> MGSSH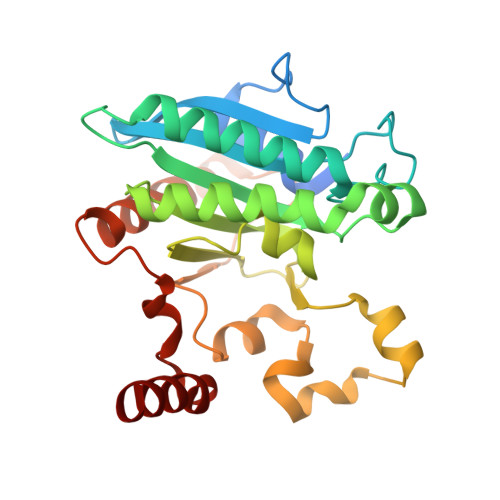HHHHHSQDPNSMSQPFASRGLAWFQALAGSLAPRPGDPASLRVADAELDGYPVRFLAVVPDPDNPFPRARQGEVGLLEGWGLAAAVDEALEADREAPRKRALLAIVDVPSQAYGRREEALGIHQALAGAVDAYARARLAGHPLIGLLVGKAMSGAFLAHGYQANRLIALHDPGVMVHAMGKAAAARITLRSVEELEALAAKVPPMAYDIDSYASLGLLWRTLPVETVEVPSTADLVRVRTCLGEALADILGGPRDLGGRLGAANREASARVRRLLREQW(2R)-2-{[FORMYL(HYDROXY)AMINO]METHYL}HEXANOIC ACID | C8 H15 N O4 | 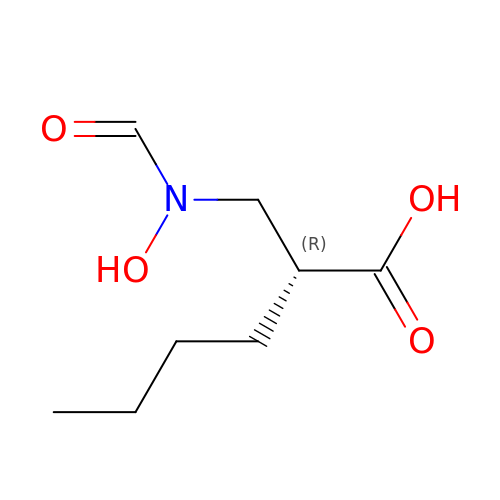NOSUUIPGNMAALM-SSDOTTSWSA-N>G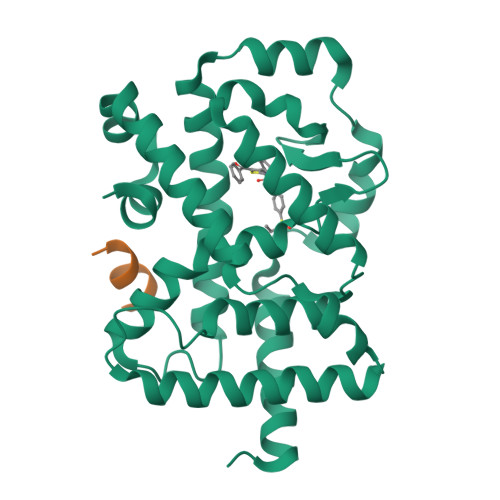PYASLTEIEHLVQSVCKSYRETCQLRLEDLLRQRSNIFSREEVTGYQRKSMWEMWERCAHHLTEAIQYVVEFAKRLSGFMELCQNDQIVLLKAGAMEVVLVRMCRAYNADNRTVFFEGKYGGMELFRALGCSELISSIFDFSHSLSALHFSEDEIALYTALVLINAHRPGLQEKRKVEQLQYNLELAFHHHLSKTHRQSILAKLPPKGKLRSLCSQHVERLQIFQHLHPIVVQAAFPPLYKELFSTETESPVGLSK[2x];>NSHQKVTLLQLLLGHKNEEN[2x]> PHMASMLEAKFEEASLFKRIIDGFKDCVQLVNFQCKEDGIIAQAVDDSRVLLVSLEIGVEAFQEYRCDHPVTLGMDLTSLSKILRCGNNTDTLTLIAD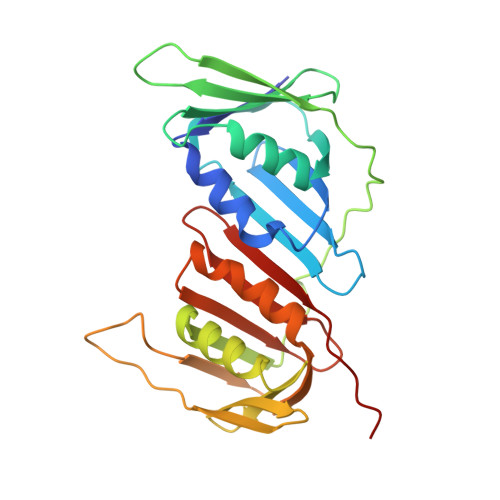NTPDSIILLFEDTKKDRIAEYSLKLMDIDADFLKIEELQYDSTLSLPSSEFSKIVRDLSQLSDSINIMITKETIKFVADGDIGSGSVIIKPFVDMEHPETSIKLEMDQPVDLTFGAKYLLDIIKGSSLSDRVGIRLSSEAPALFQFDLKSGFLQFFLAPKFNDEE>[4x]AAPEVLADFHGEMGGCDSCHVSDKGGVTNDNLTHENGQCVSCHGDLKELAAAAPKDKVSPHKSHLIGEIACTSCHKGHEKSVAYCDACHSFGFDMPFGGKWERKFVPVDADKAAQDKAIAAGVKETTDVVIIGSGGAGLAAAVSARDAGAKVILLEKEPIPGGNTKLAAGGMNAAETKPQAKLGIEDKKQIMIDDTMKGGRNINDPELVKVLANNSSDSIDWLTSMGADMTDVGR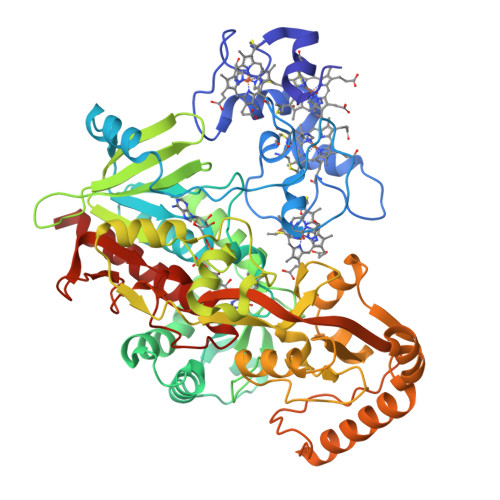MGGASVNRSHRPTGGAGVGAHVAQVLWDNAVKRGTDIRLNSRVVRILEDASGKVTGVLVKGEYTGYYVIKADAVVIAAGGFAKNNERVSKYDPKLKGFKATNHPGATGDGLDVALQAGAATRDLEYIQAHPTYSPAGGVMITEAVRGNGAIVVNREGNRFMNEITTRDKASAAILQQKGESAYLVFDDSIRKSLKAIEGYVHLNIVKEGKTIEELAKQIDVPAAELAKTVTAYNGFVKSGKDAQFERPDLPRELVVAPFYALEIAPAVHHTMGGLVIDTKAEVKSEKTGKPITGLYAAGEVTGGVHGANRLGGNAISDIVTYGRIAGASAAKFAKDN> ASQVGVIKPWLLLGSQDAAHDLDTLKKNKVTHILNVAYGVENAFLSDFTYKSISILDLPETNILSYFPECFEFIEEAKRKDG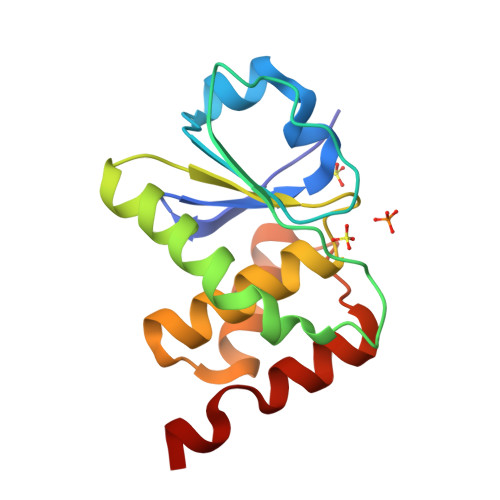VVLVHSNAGVSRAAAIVIGFLMNSEQTSFTSAFSLVKNARPSICPNSGFMEQLRTYQEGKES>[2x]NCSKIHLSTKLLAVDFPAHFVKSISCQICEHILADPVETSCKHLFCRICILRCLKVMGSYCPSCRYPCFPTDLESPVKSFLNILNSLMVKCPAQDCNEEVSLEKYNHHVSSHKESKETLVHINKGGRPRQHLLSLTRRAQKHRLRELKIQVKEFADKEEGGDVKAVCLTLFLLALRARNEHRQADELEAIMQGRGSGLQPAVCLAIRVNTFLSCSQYHKMYRTVKAITGRQIFQPLHALRNAEKVLLPGYHPFEWQPPLKNVSSRTDVGIIDGLSGLASSVDEYPVDTIAKRFRYDSALVSALMDMEEDILEGMRSQDLDDYLNGPFTVVVKESCDGMGDVSEKHGSGPAVPEKAVRFSFTVMRITIEHGSQNVKVFEEPKPNSELCCKPLCLMLADESDHETLTAILSPLIAEREAMKSSELTLEMGGIPRTFKFIFRGTGYDEKLVREVEGLEASGSVYICTLCDTTRLEASQNLVFHSITRSHAENLQRYEVWRSNPYHESVEELRDRVKGVSAKPFIETVPSIDALHCDIGNAAEFYKIFQLEIGEVYKHPNASKEERKRWQATLDKHLRKRMNLKPIMRMNGNFAR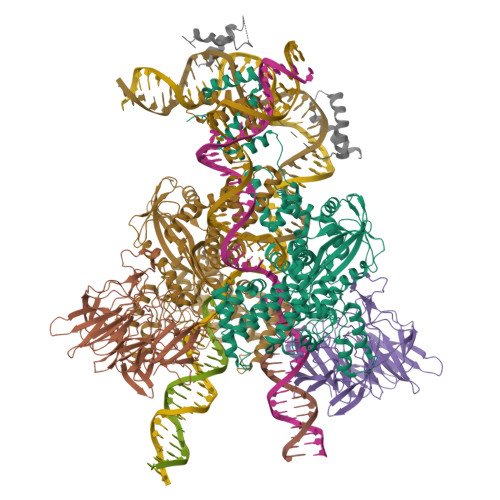KLMTQETVDAVCELIPSEERHEALRELMDLYLKMKPVWRSSCPAKECPESLCQYSFNSQRFAELLSTKFKYRYEGKITNYFHKTLAHVPEIIERDGSIGAWASEGNQSGNKLFRRFRKMNARQSKCYEMEDVLKHHWLYTSKYLQKFMNAHNALKSSGFTMNSKETLGDPLGIEDSLESQDSME;>[2x]MSLQMVTVGHNIALIQPGFSLMNFDGQVFFFGQKGWPKRSCPTGVFHFDIKQNHLKLKPAIFSKDSCYLPPLRYPATCSYKGSIDSDKHQYIIHGGKTPNNELSDKIYIMSVACKNNKKVTFRCTEKDLVGDVPEPRYGHSIDVVYSRGKSMGVLFGGRSYMPSTQRTTEKWNSVADCLPHVFLIDFEFGCATSYILPELQDGLSFHVSIARNDTVYILGGHSLASNIRPANLYRIRVDLPLGTPAVNCTVLPGGISVSSAILTQTNNDEFVIVGGYQLENQKRMVCSLVSLGDNTIEISEMETPDWTSDIKHSKIWFGSNMGNGTIFLGIPGDNKQAMSEAFYFYTLRCSEEDLSEDQKIVSNSQTSTEDPGDSTPFEDSEEFCFSAEATSFDGDDEFDTYNEDDEDDESVTGYWITCCPTCDVDINTWVPFYSTELNKPAMIYCSHGDGHWVHAQCMDLEERTLIHLSEGSNKYYCNEHVQIARALQAPKRNPPLQKPPMKSLHKKGSGKVLTPAKKS;> SYAFFVQTCREEHKKKHPDASVNFSEFSKKCSERWKTMSAKEKGKFEDMAKADKARYEREMKTYIPPKGETKKKFKDPNAPKRPPSAFFLFCSEYRPKIKGEHPGLSIGDVAKKLGEMWNNTAADD Due to the amphipathic property, S1P cannot diffuse freely but has to be transported across the cell membrane through active transport. Among these transporters, Spns2 is the first identified and the most extensively studied. Human Spns2 is a classical MFS member with twelve transmembrane (TM) helices and a molecular weight of ~58 kDa, which is small for cryo-EM analysis. Here, we reported two cryo-electron microscopy (EM) structures of human Spns2 in inward-open conformations bound to S1P or inhibitor 16d.

We determined the structure of the Spns2fusion construct at an overall resolution of 3.60 Å using cryo-EM. Notably, Spns2fusion was mainly expressed in the plasma membrane and maintained a similar S1P transport activity as the wild-type (WT) Spns2. Notably, an elongated extra density in the central cavity extends into the C-terminal domain (CTD). This density could accommodate one S1P molecule well. The affinity selection mass spectrometry results confirmed that endogenous S1P bound to Spns2fusion. The phosphoryl group of S1P forms extensive polar interactions with Spns2, specifically residues Q463 and S464 on TM11, and the amino group of S1P interacts with S326 on TM7. Compared to WT Spns2, the double and triple mutants of S326, Q463, and S464, as well as alanine substitutions of Y246 and I429, substantially decreased S1P transport activity, but other residues showed less effect. Intriguingly, several positively charged residues, including R227, R456, R119, and R200 are located around the cavity but at some distance from the S1P binding site, which may participate in S1P recognition and translocation during the dynamic transport process. Residues D118, R119, R200, and E207 form a hydrogen-bond network to stabilize the local conformation of NTD.

> MDYKDDDDKLEVLFQGPGSMMCLECASAAAGGAEEEEADAERRRRRRGAQRGAGGSGCCGARGAGGAGVSAAGDEVQTLSGSVRRAPTGPPGTPGTPGCAATAKGPGAQQPKPASLGRGRGAAAAILSLGNVLNYLDRYTVAGVLLDIQQHFGVKDRGAGLLQSVFICSFMVAAPIFGYLGDRFNRKVILSCGIFFWSAVTFSSSFIPQQYFWLLVLSRGLVGIGEASYSTIAPTIIGDLFGIDCSFWNESYLTGSRDERKKSLLSKFGMDEGVTFMFIGRFDRGQKGVDVLLKAIEILSSKKEFQEMRFIIIGKGDPELEGWARSLEEKHGNVKVITEMLSREFVRELYGSVDFVIIPSYFEPFGLVALEAMCLGAIPIASAVGGLRDIITNETGILVKAGDPGELANAILKALELSRSDLSKFRENCKKRAMSFSTKNTRTLMLSVFYFAIPLGSGLGYITGSSVKQAAGDWHWALRVSPVLGMITGTLILILVPATKRGHADQLGDQLKARTSWLRDMKALIRNRSYVFSSLATSAVSFATGALGMWIPLYLHRAQVVQKTAETCNSPPCGAKDSLIFGAITCFTGFLGVVTGAGATRWCRLKTQRADPLVCAVGMLGSAIFICLIFVAAKSSIVGAYICIFVGETLLFSNWAITADILMYVVIPTRRATAVALQSFTSHLLGDAGSPYLIGFISDLIRQSTKDSPLWEFLSLGYALMLCPFVVVLGGMFFLATALFFVSDRARAEQQVNQLAMPPASVKV> EESPFVSNPGNITGARGLTGTLRCQLQVQGEPPEVHWLRDGQILELADSTQTQVPLGEDEQGDWIVASQLRITSLQLSDTGQYQCLVFLGHQTFVSQPGYVRLEGLPYFLEEPEDRTVAANTPFNLSCQAQGPPEPVDLLWLQDAVPLATAPGHGPQRSLHVPGLNKTSSFSCEAHNAKGVTTS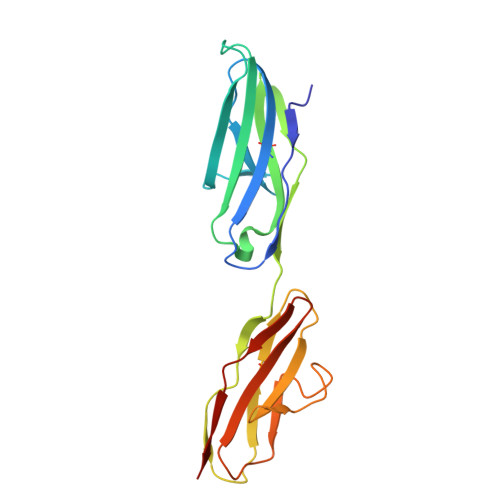RTATITVLPQQ>[4x]MGSDKIHHHHHHMNPLDLIAKRAYPYETEKRDKTYLALNENPFPFPEDLVDEVFRRLNSDALRIYYDSPDEELIEKILSYLDTDFLSKNNVSVGNGADEIIYVMMLMFDRSVFFPPTYSCYRIFAKAVGAKFLEVPLTKDLRIPEVNVGEGDVVFIPNPNNPTGHVFEREEIERILKTGAFVALDEAYYEFHGESYVDFLKKYENLAVIRTFSKAFSLAAQRVG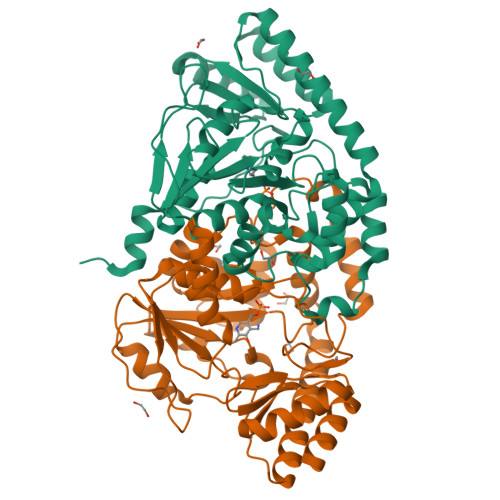YVVASEKFIDAYNRVRLPFNVSYVSQMFAKVALDHREIFEERTKFIVEERERMKSALREMGYRITDSRGNFVFVFMEKEEKERLLEHLRTKNVAVRSFREGVRITIGKREENDMILRELEVFK2-methyl-1H-benzimidazol-7-ol | C8 H8 N2 O | 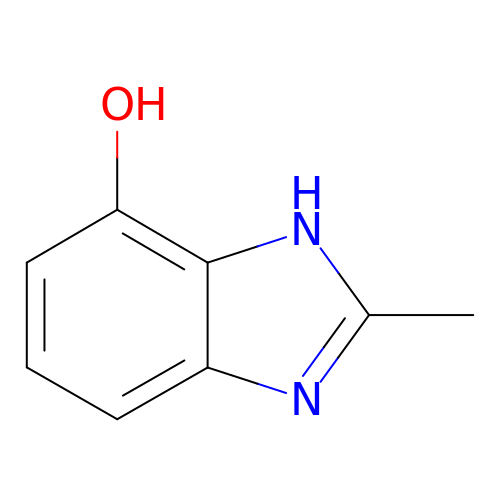HLPAESMITTURFN-UHFFFAOYSA-N{(1S)-1-(3,4-difluorophenyl)-4-[hydroxy(methyl)amino]-4-oxobutyl}phosphonic acid | C11 H14 F2 N O5 P | 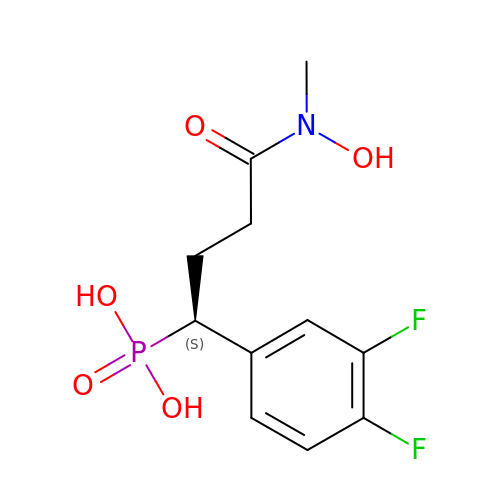IZWIBRNXHRUNKD-JTQLQIEISA-N Endo-1,4-β-glucanase from the earthworm Eisenia fetida (EF-EG2) belonging to glycoside hydrolase family 9 has been shown to have the highest activity at 313 K, and also retained a comparatively high activity at 283 K. The recombinant EF-EG2 was purified expressed in Pichia pastoris, and then grew needle-shaped crystals with dimensions of 0.02 × 0.02 × 1 mm. Recombinant EF-EG2 hydrolyzes soluble cellulose (carboxymethyl cellulose), but not insoluble (powdered cellulose) or crystalline (Avicel) cellulose substrates. The enzyme exhibited significant activity at 283 K (38% of the activity at optimal 313 K) and was stable at pH 5.0–9.0, with an optimum pH of 5.5. The overall structure of EF-EG2 has an (α/α)6 barrel fold which contains a putative active-site cleft and a negatively charged surface.

The crystal structure of EF-EG2 was determined at 1.5 Å resolution as the second example of eukaryotic GH family 9 enzyme following that of NtEgl. The crystals belonged to the space group P3221 with unit-cell parameters of a = b = 136 Å, c = 55.0 Å. The final refined EF-EG2 structure includes 435 residues (Phe21–Gly455), which have 23 alternative side-chain conformations, two ions (Ca2+ and Na+), seven crystallization reagents (one citrate, one Tris and five glycerol molecules) and 694 waters. The overall structure of EF-EG2 consists of 12 α-helices which form the (α/α)6 barrel fold, an additional six short helices and two β-strands. The location of the calcium ion is conserved in GH family 9 enzyme structures; however, its role in the catalytic activities of these enzymes is still unclear. TRS is recognized by the side-chain carboxyl oxygen atom of Glu431 via direct hydrogen bond (O—O distance: 2.6 Å) and by those of the Asp74 and Asp77 via water-mediated hydrogen bonds. These glutamic and aspartic acid residues, Glu431, Asp74 and Asp77, are conserved throughout GH family 9 enzymes, and are thought to be crucial residues for its catalytic activity. In superposed structures, the location of TRS, GOL1 and GOL2 loosely corresponded to the glucose units in subsites −1, +1 and −2, respectively. The negatively charged amino acids (Asp and Glu) of EF-EG2 occupy over two-thirds of accessible surface area (ASA) from the total charged amino acids (ASAAsp,Glu: 2900 Å2; ASAArg,Lys: 1300 Å2) whereas those of NtEgl occupy about half (ASAAsp,Glu: 2400 Å2; ASAArg,Lys: 2300 Å2). CtCelT has a slightly higher activity at 303 K than NtEgl, but almost loses activity at 293 K. Thus, it seems that the highly negatively charged surface of EF-EG2 contributes to its cold adaptation under 293 K. The increase in surface negative charge has also been described for cold-adapted cellulase belonging to GH family 5 from the Antarctic bacterium Pseudoalteromonas haloplanktis which retains sufficient activity at 297 K.

> EAEFQYNYDEVLEKSILFYEAERSGDLPANNRIPYRGDSALGDQGNQGQDLTGGWYDAGDHVKFGFPMAFATTTLAWGILEFRDGYEAAGQYNLALDSIRWTLNYFLKAHVSDNEFYGQVGDANTDHAYWGRPEDMTMERPAWSISPSAPGSDLAAETAAALAAGYLVFRDSDAAFANNLLAHSRTLYDFALNNRGIYSQSISNAAGFYASSAYEDELAWGAAWLYRATEEQEYLDRAYEFGTTTNTAWAYDWNEKIVGYQLLLTTSAGQTDFLPRVENFLRNWFPGGSVQYTPLGLAWLAQWGPNRYAANAAFIALVSAKYNILASESEQFARSQIHYMLGDAGRSYVVGFGNNPPQQPHHRSSSCPDQPAECDWDEFNQPGPNYQILYGALVGGPDQNDQFEDLRSDYIRNEVANDYNAGFQGAVAALRAIQLRDGKEQKLISEEDLNSAVDHHHHHH> TNCDREPIHIPGAIQPHGVLLVLSEPGLVLTHASENAPAVLGNSAEQLLGAPLGHFIEPSVREPLEADLRSARLKQLNPLKVVWRVDGVDRFFDGIAHRHQGRLILELEPSSHREAVPFLSFFHAVRDGLSRLRDARDLQELCEAVVQEVRGLTGFDRAIIYRFDAEWNGSVIAEARDARADPYLGLHFPASDIPRQARELYQLNWLRIIPTIDYQPARVRALPGHGEPLDLSFSVLRSVSPIHLEYLHNMGVQASMSISLMKDGKLWGLISCTQVSGTRYVPYEVRTACEFLGEVMSSLLAA

Phytochromes are red-light photoreceptors found in various plants and microorganisms. S. aurantiaca contains two previously uncharacterized bacteriophytochromes (BphPs) denoted SaBphP1 and SaBphP2, which may be responsible for the light-stimulated growth of multicellular fruiting bodies. The classical BphPs switch between a red absorbing state denoted Pr (λmax ≃ 700 nm) and a far-red absorbing state denoted Pfr (λmax ≃ 750 nm).

The SaBphP1 and other myxobacterial BphPs lack a conserved histidine (His) at position 289 in the GAF domain. In the classical BphPs, the equivalent His forms a critical hydrogen bond to the BV ring D that stabilizes the Pr state. SaBphP1 contains a threonine (Thr289) at this position, which is replaced by glycine in some myxobacterial BphPs. The wild-type and mutant CBDs both crystallize in the dark in the Pr state in space group P3221. However, the T289H mutation hardly changes the overall structure of the CBD dimer as the root-mean-square deviation (r.m.s.d.) between wild-type and mutant is on the order of 0.3 Å. Since the CBDs do not form stable Pfr spectra, but the PCMs do, the PHY domain is essential for the mechanics of the photoswitch.> MH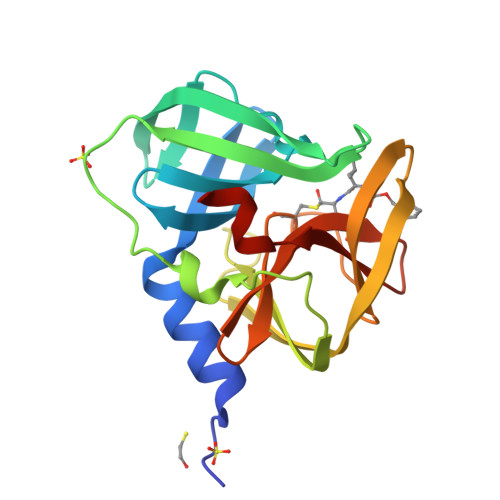HHHHHGPGFDYAVAMAKRNIVTATTSKGEFTMLGVHDNVAILPTHASPGESIVIDGKEVEILDAKALEDQAGTNLEITIITLKRNEKFRDIRPHIPTQITETNDGVLIVNTSKYPNMYVPVGAVTEQGYLNLGGRQTARTLMYNFPTRAGQCGGVITCTGKVIGMHVGGNGSHGFAAALKRSYFTQSQ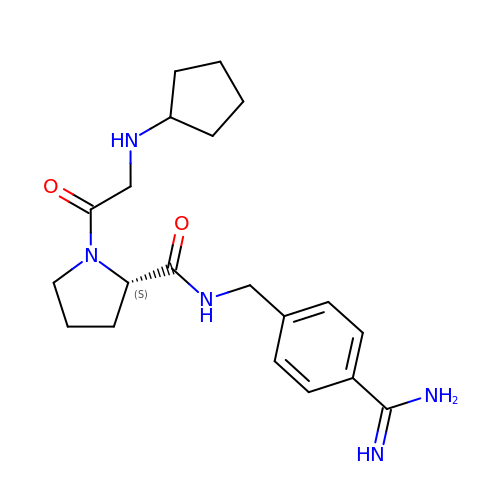(S)-N-(4-carbamimidoylbenzyl)-1-(2-(cyclopentylamino)ethanoyl)pyrrolidine-2-carboxamide | C20 H29 N5 O2 | WXYKSWZWRHMJTE-KRWDZBQOSA-N>[4x]ARTDNFKLSSLANGLKVATSNTPGHFSALGLYIDAGSRFEGRNLKGCTHILDRLAFKSTEHVEGRAMAETLELLGGNYQCTSSRENLMYQASVFNQDVGKMLQLMSETVRFPKITEQELQEQKLSAEYEIDEVWMKPELVLPELLHTAAYSGETLGSPLICPRGLIPSISKYYLLDYRNKFYTPENTVAAFVGVPHEKALELTGKYLGDWQSTHPPITKKVAQYTGGESCIPPAPVFGNLPELFHIQIGFEGLPIDHPDIYALATLQTLLGGGGSFSAGGPG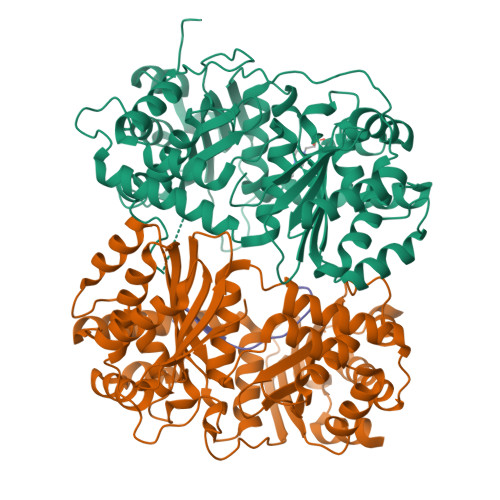KGMYSRLYTHVLNQYYFVENCVAFNHSYSDSGIFGISLSCIPQAAPQAVEVIAQQMYNTFANKDLRLTEDEVSRAKNQLKSSLLMNLESKLVELEDMGRQVLMHGRKIPVNEMISKIEDLKPDDISRVAEMIFTGNVNNAGNGKGRATVVMQGDRGSFGDVENVLKAYGLGNSSSSKNDSPKKKGWFHHHHHH;>[4x]ASQIPGTRTSKLPNGLTIATEYIPNTSSATVGIFVDAGSRAENVKNNGTAHFLQHLAFKGTQNRPQQGIELEIENIGSHLNAYTSRENTVYYAKSLQEDIPKAVDILSDILTKSVLDNSAIERERDVIIRESEEVDKMYDEVVFDHLHEITYKDQPLGRTILGPIKNIKSITRTDLKDYITKNYKGDRMVLAGAGAVDHEKLVQYAQKYFGHVPKSESPVPLGSPRGPLPVFCRGERFIKENTLPTTHIAIALEGVSWSAPDYFVALATQAIVGNWDRAIGTGTNSPSPLAVAASQNGSLANSYMSFSTSYADSGLWGMYIVTDSNEHNVRLIVNEILKEWKRIKSGKISDAEVNRAKAQLKAALLLSLDGSTAIVEDIGRQVVTTGKRLSPEEVFEQVDKITKDDIIMWANYRLQNKPVSMVALGNTSTVPNVSYIEEKLNQ;>LSLRQSIRFFKPATRTLCSSRYLL[4x]> MIAVKDITDLNIQDIISQLTSEVINGDTTPSSAKFACEINSYIINYNLSNINLI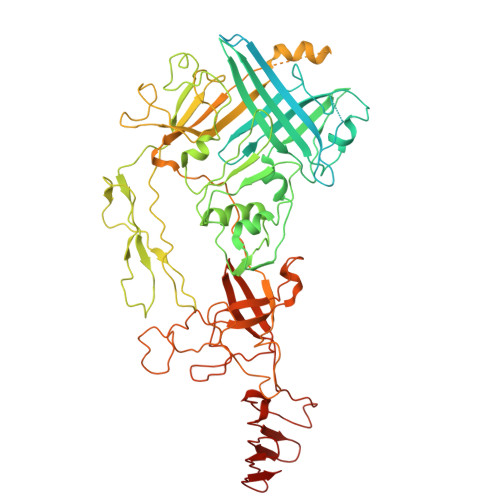NTQLKNTKILYRKGLISKLDYEKYKRYCIISRFKNNIDEFILYFSTNYKDSQSLKIAIKELQNSCSSSLILELPHDYIRKIDVLLTSIDSAIQRSSDLNKTIIKQLNKLRSSLSRYIGYNNVLQKQEITINIKPINKNFELEDISFVSTRNKQYFKHNSLTLKNPHIEKLEVCENIYGINGWLTFDLAYINNHKDFNFLLSPNQPILLDIQINDSFNFYKKESKKDHHKRTTRFIAIGFNSNSIDIHENFEYSIYSYTKNVSSGVKKFKIQFHDPLKALWTKHKPSYIALNKSLDDIFKDNFFFDSLFSLDTNKSNNLKIRIPQAFISTVNRNFYDFFIQQLEQNKCYLKYFCDKKSGKVSYHVVDQVDNDLQRNIVNSDEDLKDKLSPYDISCFKKQILISNKSNFYVKEKNICPDVTLNTQRKEDRKISDTLVKPFSSILKDNLQSVEYIQSNNDDKQEIITTGFEILLTSRNTLPFLDTEITLSKLDNDQNYLLGATDIKSLYISQRKLLFKRSKYCSKQLYENLHNFHYKSDSESDVYEKIAFTKYPSLTHDNSITYKIKDYSNLTPEYPKYKSFSNFYINGRITIGENVNNDSKKAYKFFKNHKPEESSIAEFQENGEKGTSAILNSKADILYAIEIAKEMLSDKSSDKPIIYLPLKVNINSANNQFIPLRNDDIILIEIQSFTKGEIIELISNSAISTKKAQQQLLQRQLLGSKENCEMAYTQTSDSETFSLTQVNEDCENSFLINDKKGIFLRYKSKGN>SNAAVAEVVRVQLDVKFDFDKSKVKENSYADIKNLADFMKQYPSTSTTVEGHTDSVGTDAYNQKLSERRANAVRDVLVNEYGVEGGRVNAVGYGESRPVADNATAEGRAINR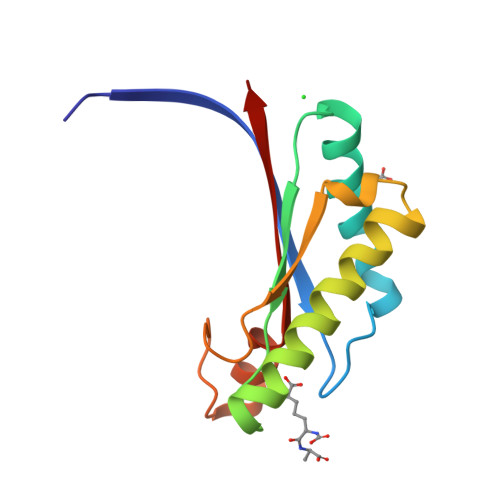RVEAEVEAEAK[4x]>[4x]MKKYRVQPDGRFELKRFDPDDTSAFEGGKQAALEALAVLNRRLEKLQELLYAEGQHKVLVVLQAMDAGGKDGTIRVVFDGVNPSGVRVASFGVPTEQELARDYLWRVHQQVPRKGELVIFDRS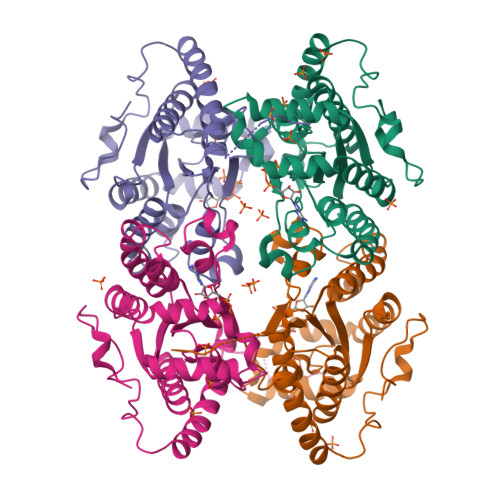HYEDVLVVRVKNLVPQQVWQKRYRHIREFERMLADEGTTILKFFLHISKDEQRQRLQERLDNPEKRWKFRMGDLEDRRLWDRYQEAYEAAIRETSTEYAPWYVIPANKNWYRNWLVSHILVETLEGLAMQYPQPETASEKIVIE> SNAMILITGANGQLGTELRYLLDERNEEYVAVDVAEMDIIDAEMVEKVFEEVKPTLVYHCAAYTAVDAAEDEGKELDFAINVTGTKNVAKASEKHGATLVYISTDYVFDGKKPVGQEWEVDDRPDPQTEYGRTKRMGEELVEKHVSNFYIIRT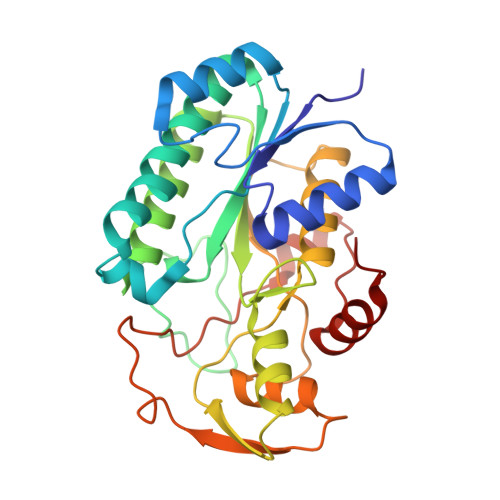AWVFGNYGKNFVFTMQNLAKTHKTLTVVNDQYGRPTWTRTLAEFITYLAENRKEFGYYHLSNDATEDTTWYDFAVEILKDTDVEVKPVDSSQFPAKAKRPLNSTMSLAKAKATGFVIPTWQDALQEFYKQEVR>[2x]PVFAKAIQKRV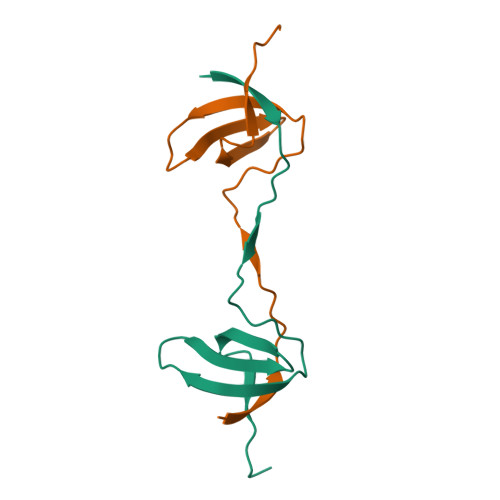PCAYDKTALALEVGDIVKVTRMNINGQWEGEVNGRKGLFPFTHVKIFDPQNPDENE>MSKEYHIDEEVGFALPNPQENLPDFYNDWMFIAKHLPDLIESGQLRERVEKLNMLSIDHLTDHKSQRLARLVLGCITMAYVWGKGHGDVRKVLPRNIAVPYCQLSKKLELPPILVYADCVLANWKKKDPNKPLTYENMDVLFSFRDGDCSKGFFLVSLLVEIAAASAIKVIPTVFKAMQMQERDTLLKALLEIASCLEKALQVFHQIHDHVNPKAFFSVLRIYLSGWKGNPQLSDGLVYEGFWEDPKEFAGGSAGQSSVFQCFDVLLGIQQTAGGGHAAQFLQDMRRYMPPAHRNFLCSLESNPSVREFVLSKGDAGLREAYDACVKALVSLRSYHLQIVTKYILIPASQQ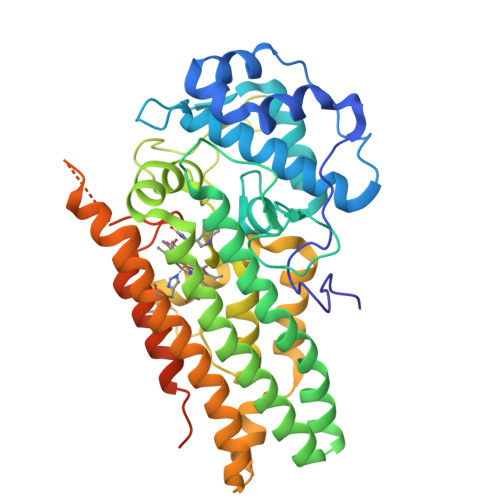PKENKTSEDPSKLEAKGTGGTDLMNFLKTVRSTTEKSLLKEGKGELNSKLEGKPIPNPLLGLDSTRTGHHHHHH[2x]>YGPDQRAQKKGDIILGGLFPIHFGVAAKDQDLKSRPESVECIRYNFRGFRWLQAMIFAIEEINSSPALLPNLTLGYRIFDTCNTVSKALEATLSFVAQNKIDSLNLDEFCNCSEHIPSTIAVVGATGSGVSTAVANLLGLFYIPQVSYASSSRLLSNKNQFKSFLRTIPNDEHQATAMADIIEYFRWNWVGTIAADDDYGRPGIEKFREEAEERDICIDFSELISQYSDEEEIQHVVEVIQNSTAKVIVVFSSGPDLEPLIKEIVRRNITGKIWLASEAWASSSLIAMPQYFHVVGGTIGFALKAGQIPGFREFLKKVHPRKSVHNGFAKEFWEETFNCHLQEGAKGPLPVDTFLRGHEESGDRFSNSSTAFRPLCTGDENISSVETPYIDYTHLRISYNVYLAVYSIAHALQDIYTCLPGRGLFTNGSCADIKKVEAWQVLKHLRHLNFTNNMGEQVTFDECGDLVGNYSIINWHLSPEDGSIVFKEVGYYNVYAKKGERLFINEEKILWSGFSREVPFSNCSRDCLAGTRKGIIEGEPTCCFECVECPDGEYSDETDASACNKCPDDFWSNENHTSCIAKEIEFLSWTEPFGIALTLFAVLGIFLTAFVLGVFIKFRNTPIVKATNRELSYLLLFSLLCCFSSSLFFIGEPQDWTCRLRQPAFGISFVLCISCILVKTNRVLLVFEAKIPTSFHRKWWGLNLQFLLVFLCTFMQIVICVIWLYTAPPSSYRNQELEDEIIFITCHEGSLMALGFLIGYTCLLAAICFFFAFKSRKLPENFNE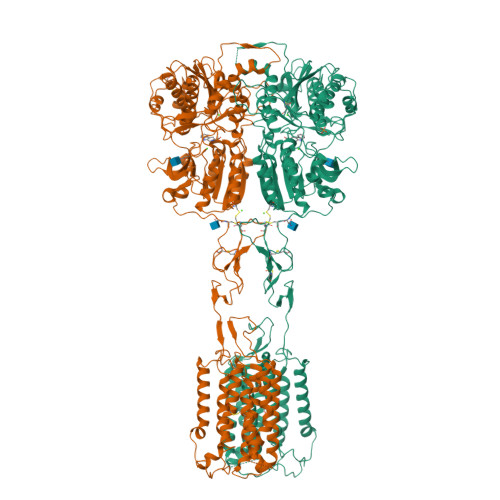AKFITFSMLIFFIVWISFIPAYASTYGKFVSAVEVIAILAASFGLLACIFFNKIYIILFKPSRNTIEAAADYKDDDDK[2x]>KAFAKFPSSASISPNPFTVSIPDEQLDDLKTLVRLSKIAPPTYESLQADGRFGITSEWLTTMREKWLSEFDWRPFEARLNSFPQFTTEIEGLTIHFAALFSEREDAVPIALLHGWPGSFVEFYPILQLFREEYTPETLPFHLVVPSLPGYTFSSGPPLDKDFGLMDNARVVDQLMKDLGFGSGYIIQGGDIGSFVGRLLGVGFDACKAVHLNLCAMRAPPEGPSIESLSAAEKEGIARMEKFMTDGLAYAMEHSTRPSTIGHVLSSSPIALLAWIGEKYLQWVDKPLPSETILEMVSLYWLTESFPRAIHTYRETTPTASAPNGA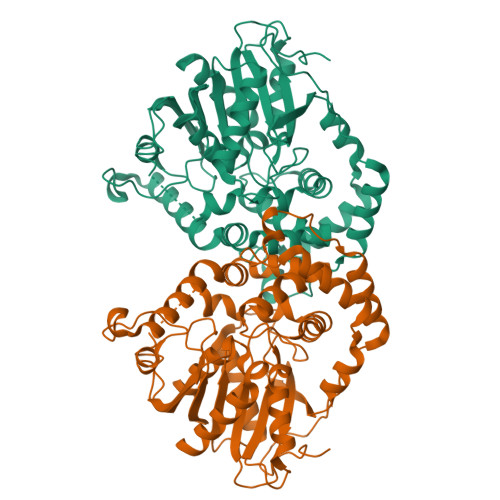TMLQKELYIHKPFGFSFFPKDLCPVPRSWIATTGNLVFFRDHAEGGHFAALERPRELKTDLTAFVEQVW[2x]> XGQLKKIAKQLKKIAYQLKKIAQ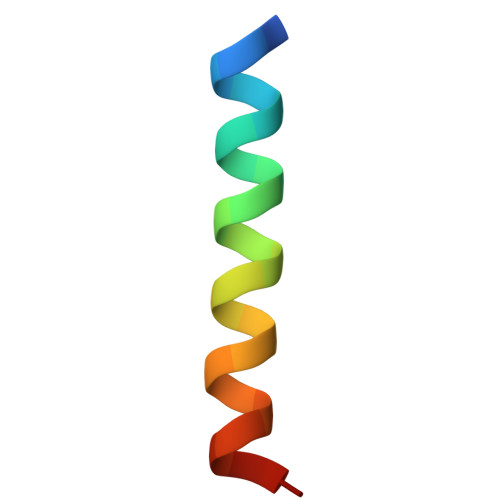GX> GHMAPGQKECDNALRQLETVRELLENPVQPINDMSYFGCLDSVMENSKVLGEAMTGISQNAKNGNLPEFGDAIATASKALCGFTEAAAQAAYLVGVSDPNSQAGQQGLVEPTQFARANQAIQMACQSLGEPGCTQAQVLSAATIVAKHTSALCNSCRLASARTANPTAKRQFVQSAKEVANSTANLVKTIKALDGDFTEENRAQCRAATAPLLEAVDNLSAFASNPEFSS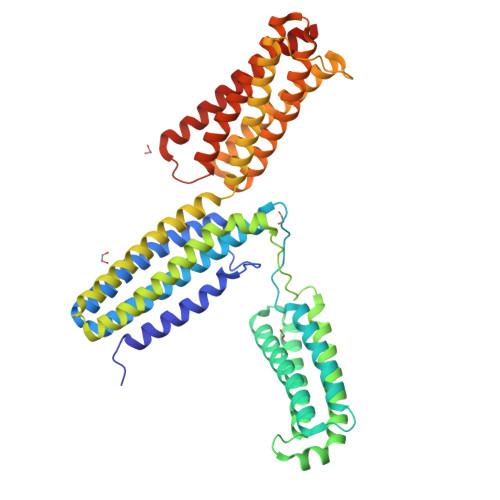VPAQISPEGRAAMEPIVISAKTMLESAGGLIQTARALAVNPRDPPRWSVLAGHSRTVSDSIKKLITSMRDKAPGQLECETAIAALNSCLRDLDQASLAAVSQQLAPREGISQEALHTQMLTAVQEISHLIEPLASAARAEASQLGHKVSQMAQYFEPLTLAAVGAASKTLSHPQQMALLDQTKTLAESALQLLYTAKEAGGNPKQAAHTQEALEEAVQMMTEAVEDLTTTLNEAASAAG> GUCUAAAGUUUGCU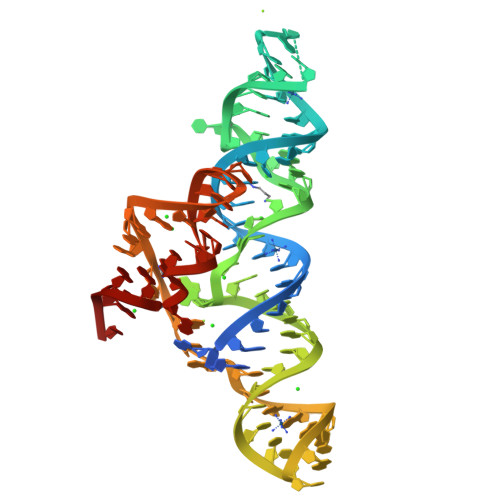AGGGUUCCGCGUCAUAGGUGGUCUGGUCCAAGAGCAAACGGCUUUCACAAAGCCACACGGAAGGAUAAAAGCCUGGGAGAU> LGRTTRDDLINGNSASCRDVIFIYARGSTETGNLGTLGPSIASNLESAFGKDGVWIQGVGGAYRATLGDNALPRGTSSAAIREMLGLFQQANTKCPDATLIAGGYSQGAALAAASIED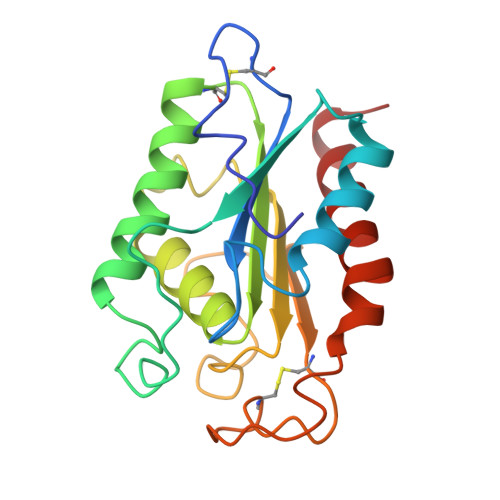LDSAIRDKIAGTVLFGYTKNLQNRGRIPNYPADRTKVFCNTGDLVCTGSLIVAAPHLAYGPDARGPAPEFLIEKVRAVRGSA>[4x]SMTSSGSSRDLFRALNSFIQTPTLPPPADLDAIISSYLERHDKPEEGSGDRLNDELLAIWDKAVQDHPEKYAAFVAVLRQLRPGLGAPARTFQWWDKLLDPVLDNATREKGLARSFMDFTLEILSSSEYDDPEAWGEEGFIPWLNRLLVRWMELRESRADFRPSTDLKEQVLTDALLAFGKKDPKGFMNALNAFVLRREHRNSAFSLLCAFVNSGPPHLYLIL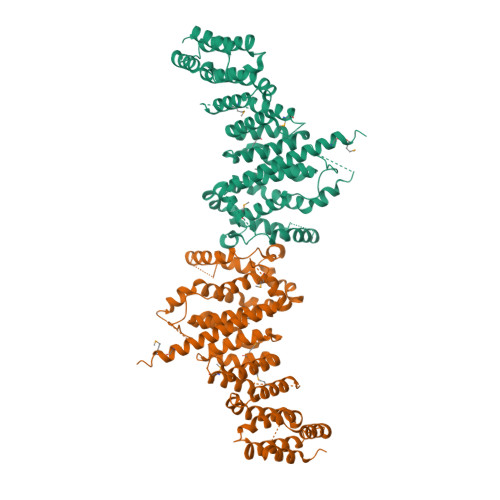QTPLFGNILQSLQKDESTFTVNLALIALVMLLPFFPGDIVPYLPTLFNIYARLLFWDRDSYFAQQHTEMGENHGESGTDTPWDKVLLDPDYDGHSVPYLPEYFTILYGLYPINFVDYIRKPHNYLPHAGSDDDIDVHAAEIRERSERFRKQHLLHPNFYEYTIETEKTNITRWLKSEADEIIADCMALVVDRGTADESRPGVEIIEQVSLLRYQRHRLLNDLQYERFVRQQHMSHMGELRRRQ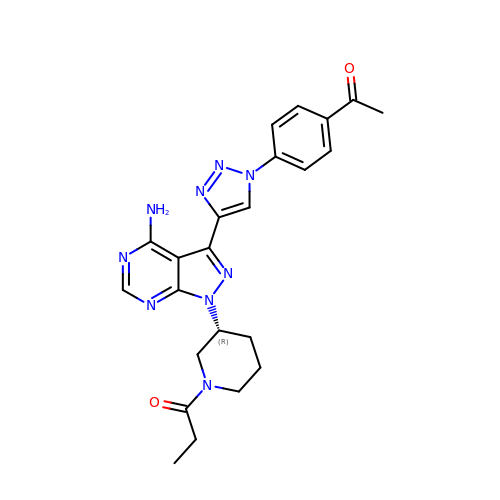1-[(3~{R})-3-[4-azanyl-3-[1-(4-ethanoylphenyl)-1,2,3-triazol-4-yl]pyrazolo[3,4-d]pyrimidin-1-yl]piperidin-1-yl]propan-1-one | C23 H25 N9 O2 | DMPCFHLMZNTFEB-QGZVFWFLSA-N> GAVEEDDKDKAKRVSRNKSEKKRRDQFNVLIKELGSMLPGNARKMDKSTVLQKSIDFLRKHKETTAQSDASEIRQDWKPTFLSNEEFTQLMLEALDGFFLAIMTDGSIIYVSESVTSLLEHLPSDLVDQSIFNFIPEGEHSEVYKILSTHLLESDSLTPEYLKSKNQLEFCCHMLRGTIDPKEPSTYEYVRFIGNFKSLTSVSTSTHNGFEGTIQRTHRPSYEDRVCFVATVRLATPQFIKEMCTVEEPNEEFTSRHSLEWKFLFLDHRAPPIIGYLPFEVLGTSGYDYYHVDDLENLAKCHEHLMQYGKGKSCYYRFLTKGQQWIWLQTHYYITYHQWNSRPEFIVCTHTVVSYAEVRAE;> MEYAEHQGRIKNAREAHSQIEKRRRDKMNSFIDELASLVPTCNAMSRKLDKLTVLRMAVQHMKTLRGATNPYTEANYKPTFLSDDELKHLILRAADGFLFVVGCDRGKILFVSESVFKILNYSQNDLIGQSLFDYLHPK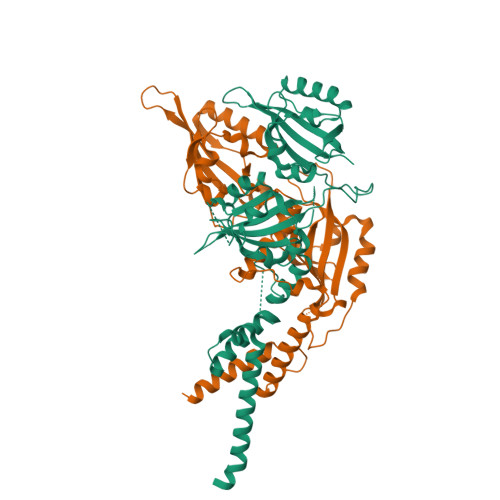DIAKVKEQLSSSDTAPRERLIDAKTGLPVKTDITPGPSRLCSGARRSFFCRMKCNRPSVKVEDKDFASTCSKKKADRKSFCTIHSTGYLKSWPPTKMGLDEDNEPDNEGCNLSCLVAIGRLHSHMVPQPANGEIRVKSMEYVSRHAIDGKFVFVDQRATAILAYLPQELLGTSCYEYFHQDDIGHLAECHRQVLQTREKITTNCYKFKIKDGSFITLRSRWFSFMNPWTKEVEYIVSTNTVVLANVLE>MKMASNDAAPSNDGAAGLVPEINHEVMAIEPVAGASLAAPVVGQLNIIDPWIRNNFVQAPAGEFTVSPRNAPGEFLLDLELGPELNPYLAHLARMYNGHAGGMEVQIVLA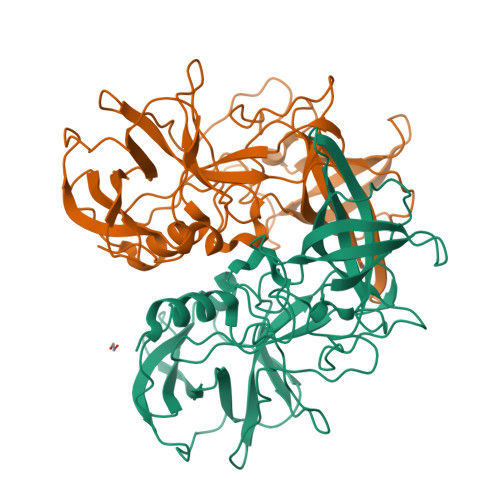GNAFTAGKILFAVIPPGFPYENLSPAQLTMCPHVVVDVRQLEPILLPMPDIRNTFFHYNQSNGPKRRLVAMLYTPLRANNAGDDVFTVSCRVLTRPSPDFEFNFLVPPSVESKTKAFTLPVLKISEMTNSRFPIPVDQMYTSRNENIVVQPQNGRVTLDGELQGTTTLQPVSICGFRGTLQTRLADQPNYTYQVHLENLDGSPVDPTDEVPAPLGTPDFQAQLFGVISQRSSDNATRAHEARVNTNDPTFAPQIAQVRFKSPSTDFSDNEPIKFTPVGISVDSQNSYNQWLLPRYGGHLTNNTHLAPSVSPMFPGEQILFFRSFMPGAGGFTDGAIDCLLPQEWVAHFYQEAATAQTDVALIRFVNPDTGRVLFEGKLHKQGFITISNSGDHPIVMPANGYFRFEAWVKQFYSLAPVGTGSGRRRVQ[2x]>[3x]QIPASEQETLVRPKPLLLKLLKSVGAQKDTYTMKEVLFYLGQYIMTKRL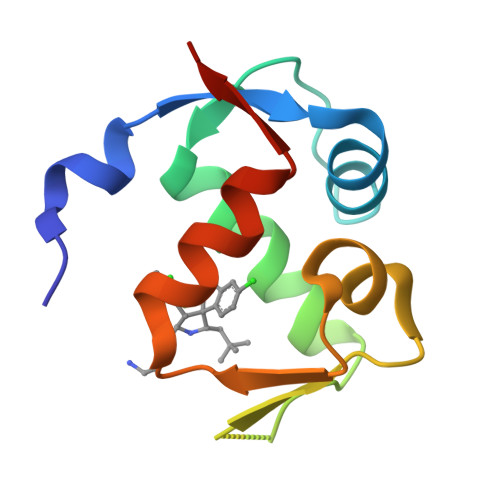YDEKQQHIVYCSNDLLGDLFGVPSFSVKEHRKIYTMIYRNLVVVNGS> MAHHHHHHMSNSDAAHAFWSTQPVPQTEDETEKIVFAGPMDEPKTVADIPEEPYPIASTFEWWTPNMEAADDIHAIYELLRDNYVEDDDSMFRFNYSEEFLQWALCPPNYIPDWHVAVRRKADKKLLAFIAGVPVTLRMGTPKYMKVKAQERGEGEEAAKYDEPRHICEINFLCVHKQLREKRLAPILIKEATRRVNRTNVWQAVYTAGVLLPTPYASGQYFHRSLNPEKLVEIRFSGIPAQYQKFQNPMAMLKRNYQLPSAPKNSGLREMKPSDVPQVRRILMNYLDSFDVGPVFSDAEISHYLLPRDGVVFTYVVENDKKVTDFFSFYRIPS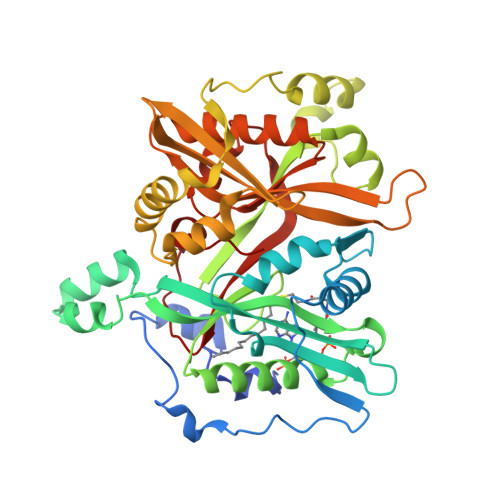TVIGNSNYNLLNAAYVHYYAATSIPLHQLILDLLIVAHSRGFDVCNMVEILDNRSFVEQLKFGAGDGHLRYYFYNWAYPKIKPSQVALVML> MSRSKRDNNFYSVEIGDSTFTVLKRYQNLKPIGSGAQGIVVAAYDAILERNVAIKKLSRPFQNQTHAKRAYRELVLMKVVNHKNIIGLLNVFTPQKSLEEFQ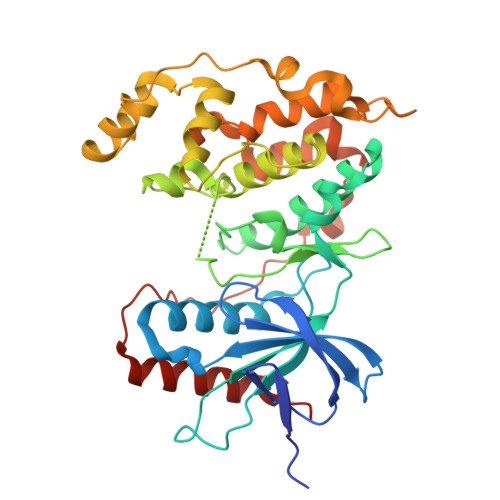DVYIVMELMDANLSQVIQMELDHERMSYLLYQMLVGIKHLHSAGIIHRDLKPSNIVVKSDATLKILDFGLARTAGTSFMMTPYVVTRYYRAPEVILGMGYKENVDIWSVGVIMGEMIKGGVLFPGTDHIDQWNKVIEQLGTPSPEFMKKLQPTVRTYVENRPKYAGYSFEKLFPDVLFPADSEHNKLKASQARDLLSKMLVIDASKRISVDEALQHPYINVWYDPSEAEAPPPKIPDKQLDEREHTIEEWKELIYKEVMDLEHHHHHH5-IMINO-4-(3-TRIFLUOROMETHYL-PHENYLAZO)-5H-PYRAZOL-3-YLAMINE 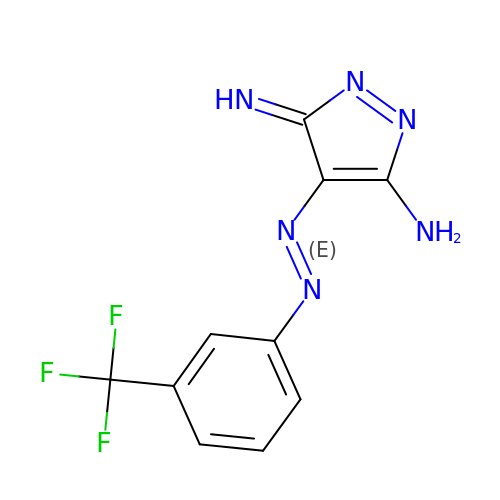| C10 H7 F3 N6 | SNTJRGVKGCPNBK-KGQVPBNKSA-N>[2x]MTASTVAACGSD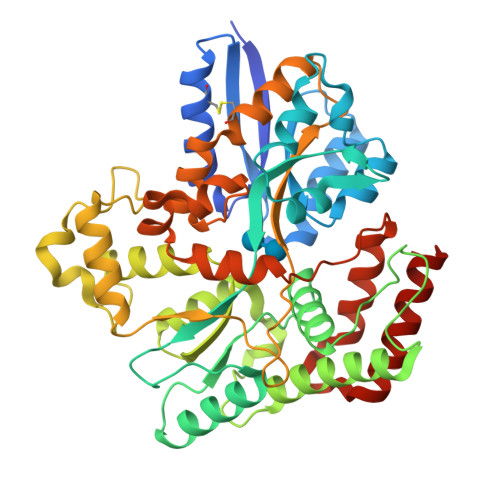SGEIVISYYTPANEAATFTAVAQRCNAELGGRFRIEQRSLPREADAQRLQLARRLTGNDRSLDVMALDVVWTAEFAEAGWALPLSEDPAGLAEADATTNTLPGPLETAKWNGELYAAPITTNTQLLWYRADLMDEPPATWDEMLSEAARLHAQGGPSWIAVQGKQYEGLVVWFNTLLESAGGQVLSDDGQRVTLTDTPEHRAATVKALEIIKAVATAPGADPSITQTDENTARLALEQGRAALEVNWPYVLPSLLENAIKGGVGFLPLNENPALRGSINDVGTFAPTDEQFDLALNASKEVFGFARYPGVRPDEPARVTLGGLNLAVASTTRHKAEAFEAVRCLRNEENQRLTSIEGGLPAVRTSLYDDPQFQAKYPQYEIIRDQLINAAVRPATPVYQAMSTRMSATLAPISQIDPERTADELAEQVQQAIDGKGLIP> AATQQEIMKNMWDPFQSMRAVTGLMELTSGQCTQLSKDAAAILAGVKESHDSISVDKNYKVLNDEVAYHAANIDAAAKANDLEEVQVQFRRMTIACRNCHKIYKTEQRLVP;> LNEHTAGDTTKSPYTIYAGL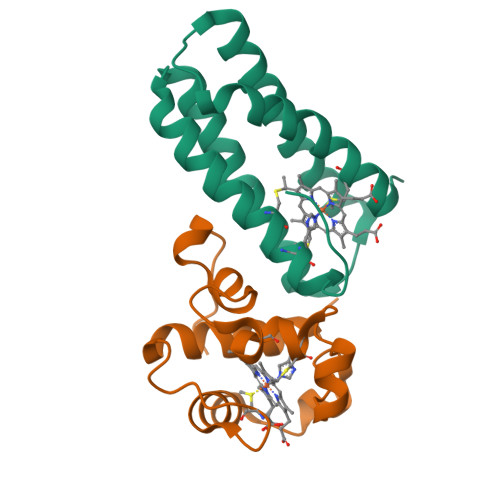GFAVQESCYYCHGNGGKGTTEGLIFGVPDFTSTEFQSSMTDKQIIDHINKGKGKMPSYQGKMSPEMIEKMAGVVRNFAVK(S)-PARA-NITROSTYRENE OXIDE | C8 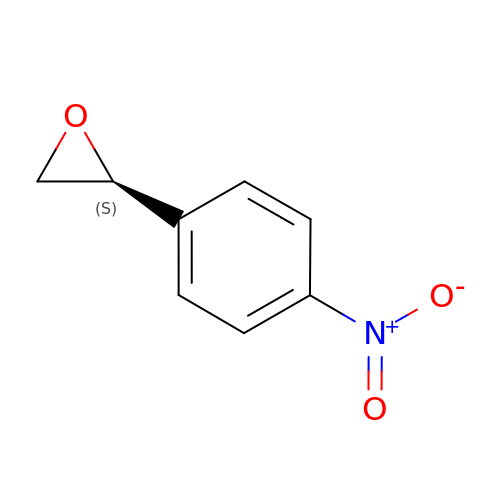H7 N O3 | YKIUTLHCSNCTDZ-MRVPVSSYSA-N>ETGRGCPTHCHCEPDGRMLLRVDCSDLGLSELPSNLSVFTSYLDLSMNNISQLLPNPLPSLRFLEELRLAGNALTYIPKGAFTGLYSLKVLMLQNNQLRHVPTEALQNLRSLQSLRLDANHISYVPPSCFSGLHSLRHLWLDDNALTEIPVQAFRSLSALQAMTLALNKIHHIPDYAFGNLSSLVVLHLHNNRIHSLGKKCFDGLHSLETLDLNYNNLDEFPTAIRTLSNLKELGFHSNNIRSIPEKAFVGNPSLITIHFYDNPIQFVGRSAFQHLPELRTLTLNGASQITEFPDLTGTANLESLTLTGAQISSLPQTVCNQLPNLQVLDLSYNLLEDLPSFSVCQKLQKIDLRHNEIYEIKVDTFQQLLSLRSLNLAWNKIAIIHPNAFSTLPSLIKLDLSSNLLSSFPITGLHGLTHLKLTGNHALQSLISSENFPELKVIEMPYAYQCCAFGVCENNGNNGDSVQCSPSGTHHHHHHHHHH[2x];>ETGICKGCLSCSKDNGCSRCQQKLFFFLRREGMRQYGECLHSCPSGYYGHRAPDMNRCARCRIENCDSCFSKDFCTKCKVGFYLHRGRCFDECPDGFAPLDETMECVEGTHHHHHHHHHH[2x]

In contrast, R-spondins (Rspo1-4) are the sole secreted potentiators of Wnt signalling and have emerged as crucial regulators of stem cell maintenance in vivo and in vitro. At the level of molecular mechanism Rspo proteins potentiate Wnt signalling by alleviating the feedback inhibition effected by the transmembrane E3 ligases ZNRF3 and RNF43. Although necessary, binding of Rspo to the E3 ectodomains is not sufficient to stop ubiquitination of Frizzled and enhance Wnt signalling. This further requires simultaneous binding of Rspo to the large leucine-rich repeat (LRR) containing ectodomain of LGR receptors 4, 5 or 6, which are well established GPCR-like regulators of stem cell function. The ternary complex between Rspo and its two receptors LGR4-6 and ZNRF3/RNF43 is established via extracellular recognition and triggers by an unknown mechanism its rapid internalisation.

To provide insight into recognition of Rspo2 by LGR receptors we crystallised a variant of the hLGR5 ectodomain (from which an unstructured loop had been removed) in complex with the Furin tandem repeat of mRspo2. The crystal structure was solved at 2.2 Å and refined to Rwork and Rfree values of 20.9% and 26.0%. The asymmetric unit contains two copies of the hLGR5ecto–mRspo2Fu1-Fu2 complex, which are essentially identical (r.m.s.d. of 0.5 Å for 559 aligned Cα). At the core of the interface is a hydrophobic interaction site with the hallmark ‘phenylalanine clamp’, in this example F105 and F109 of Rspo2Fu2 pinching A190 of hLGR5. These conserved hydrophobic core interactions are surrounded by more polar interactions which differ in a subtle way from the hLGR5–hRSPO1 interface (not all shown in figures): The side chain of N123 is found to form a hydrogen bond with H76, an interaction that was not previously seen. The salt bridge seen between R144 of LGR5 and D85 of hRSPO1 is replaced with a water-mediated hydrogen bond to the backbone of C78 of mRspo2. We observe the exact same dimeric arrangement with a twofold rotational symmetry in our structure as that seen by Peng et al.. The LGR5–LGR5 interface buries some 900 Å of solvent accessible area. Residues I293, Q294, F295, F301 and Q302 function as hinge regions mediating a domain rotation of 9.6° around an axis approximately perpendicular to the horseshoe fold. The structure described here represents the most tightly curved or concave conformation observed to date for the LGR5 ectodomain.>MDYKDDDDKGEDGKPVWAPHPTDGFQVGNIVRRGPDSLTIEPLNQKGKTFLALINQVFPAEEDSKKDVEDNCSLMYLNEATLLHNIKVRYSKDRIYTYVANILIAVNPYFDIPKIYSSETIKSYQGKSLGTMPPHVFAIADKAFRDMKVLKLSQSIIVSGESGAGKTENTKFVLRYLTESYGTGQDIDDRIVEANPLLEAFGNAKTVRNNNSSRFGKFVEIHFNEKSSVVGGFVSHYLLEKSRICVQGKEERNYHIFYRLCAGASEDIRERLHLSSPDNFRYLNRGCTRYFANKETDKQILQNRKSPEYLKAGSLKDPLLDDHGDFIR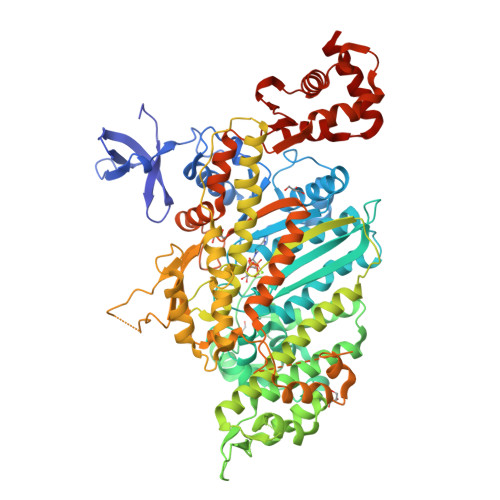MCTAMKKIGLDDEEKLDLFRVVAGVLHLGNIDFEEAGSTSGGCNLKNKSTQALEYCAELLGLDQDDLRVSLTTRVMLTTAGGAKGTVIKVPLKVEQANNARDALAKTVYSHLFDHVVNRVNQCFPFETSSYFIGVLDIAGFEYFEHNSFEQFCINYCNEKLQQFFNERILKEEQELYQKEGLGVNEVHYVDNQDCIDLIEARLVGILDILDEENRLPQPSDQHFTSAVHQKHKDHFRLSIPRKSKLAIHENIRDDEGFIIRHFAGAVCYETTQFVEKNNDALHMSLESLICESRDKFIRELFESSTNNNKDTKQKAGKLSFISVGNKFKTQLNLLLDKLRSTGASFIRCIKPNLKMTSHHFEGAQILSQLQCSGMVSVLDLMQGGFPSRASFHELYNMYKKYMPDKLARLDPRLFCKALFKALGLNEIDYKFGLTKVFFRPGKFAEFDQIMKSDPDHLAELVKRVNHWLI[2x]>SMDKPSFVIQSKEAESAAKQLGVSVIQLLPSLVKPAQSYARTPISKFNVAVVGLGSSGRIFLGVNVEFPNLPLHHSIHAEQFLVTNLTLNGERHLNFFAVSAAPCGHCRQFLQEIRDAPEIKILITDPNNSADSDSAADSDGFLRLGSFLPHRFGPDDLLGKDHPLLLESHDNHLKISDLDSICN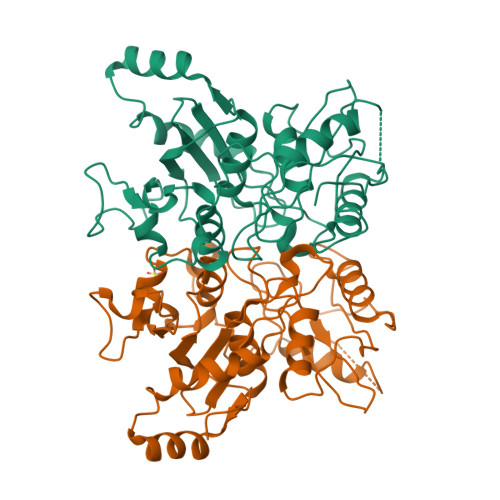GNTDSSADLKQTALAAANRSYAPYSLCPSGVSLVDCDGKVYRGWYMESAAYNPSMGPVQAALVDYVANGGGGGYERIVGAVLVEKEDAVVRQEHTARLLLETISPKCEFKVFHCYEAHHHHHH[2x]> GDVAAGASVFSANCAACHMGGR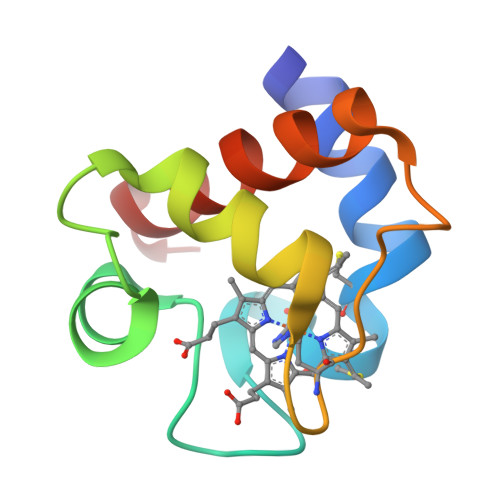NVIVANKTLSKSDLAKYLKGFDDDAVAAVAYQVTNGKNAMPGFNGRLSPLQIEDVAAYVVDQAEKGW> MHHHHHHSSGRENLYFQGEHYDVIILGTGLKECILSGLLSHYGKKILVLDRNPYYGGETASLNLTNLYNTFKPKENIPSKYGENRHWNVDLIPKFILVGGNLVKILKKTRVTNYLEWLVVEGSYVYQHQKKGFLTSEKFIHKVPATDMEALVSPLLSLMEKNRCKNFYQYVSEWDANKRNTWDNLDPYKLTMLEIYKHFNLCQLTIDFLGHAVALYLNDDYLKQPAYLTLERIKLYMQSISAFGKSPFIYPLYGLGGIPEGFSRMCAINGGTFMLNKNVVDFVFDDDNKVCGIKSSDGEIAYCDKVICDPSYVMHLKNKIKKIGQVIRCICILSNPIPETNQTNSCQIIIPQNQLNRKS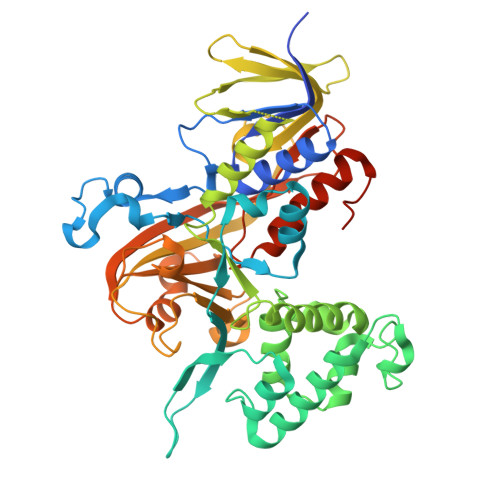DIYINLVSFQHGVTLKGKYIAIVSATVETNNPIKEIEKPLELLGTIEEKFVKISDLYVSTSKKPADNIFVTSSYDATSHFETATNDLLQIWENLWGQKLNFDDLNTNADGEAPDFN> RQNLQMEIKITTVIQHVFQNLILGSKVNWAEDPALKEIVL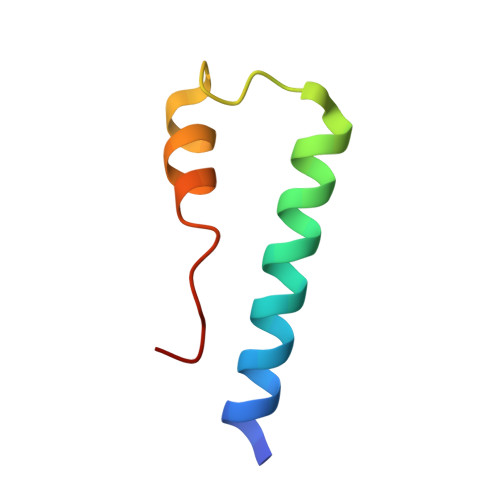QLEKNVDMM DUX4, a member of homeobox protein family, is exclusively found in placental mammals. Compared to other homeobox proteins, DUX4 contains two adjacent HD1 and HD2 domain, connected by a short linker of 15 residues. Very recently, using next-generation sequencing technologies, a novel B-ALL oncogenic driver DUX4/IGH, derived from the insertion of chromosome fragments containing DUX4 gene into the IGH locus, has been reported in ~7% of B-ALL patients. In order to investigate how DUX4/DUX4 fusions recognize DNA, we have determined the crystal structures of Apo-DUX4HD2 and DNADRE-bound complex at the resolutions of 1.5 and 2.6 Å, respectively.

In the asymmetric unit (ASU), it contains two HD2 molecules and a DNA duplex of TAATCTAAT (DRE) sequence. The HD2-DNA complex structure reveals a clamp-like DNA-binding mechanism, in which the N-terminal R95RKR98 loop and the α3 helix interact with the TAAT site in the minor and major grooves, respectively. In the minor groove, the N-terminal R95RKR98 loop adopts an extended configuration making loosen interaction with the DNA backbone. Upon DNA binding, Arg96/Lys97 or Arg95/Lys97 are utilized to make direct contract with the phosphate groups of DNA backbone in the minor groove. In the major groove, the α3 helix forms direct hydrogen bonds with DNA. Compared with the Apo-DUX4HD2 structure, the guanidinium head group of Arg137 in the DNA-bound complex shifts 2.9 Å upward to form two direct hydrogen bonds with the phosphate groups in the DNA backbone. Inside the DNA major groove lie the residues Gln143, Asn144, and Arg148, termed QNR motif. The side-chains of these residues insert deep into the major groove reading the “barcode” of T1A2A3T4. The carboxamide head group of Asn144 rotates 30° anti-clockwise to make two direct hydrogen bonds with the A2 nucleotide. In a concerted fashion, the guanidinium head group of Arg148 swings 5.3 Å into the major groove to form hydrogen bonds with the A3 site.

>GSHMGRRKRTAVTGSQTALLLRAFEKDRFPGIAAREELARETGLPESRIQIWFQNRRARHPGQG[2x]>[10x]MKSLMKPNIKRVINATGVVINTNLGRAPLSKDVINFISEIANGYSNLEYNLEEGKRGSRIAHIEKYLNELTGAESSFVVNNNAGAVFLVLNTLA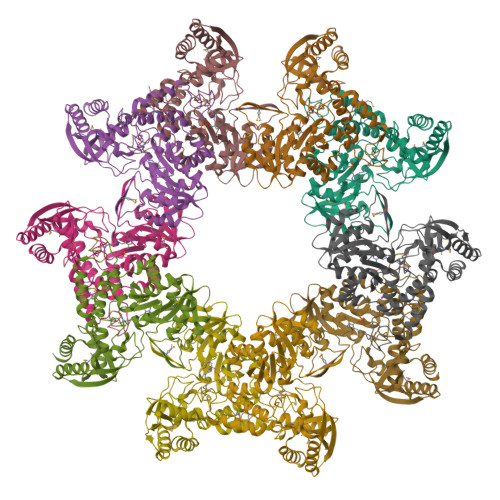EGKEVIISRGELVEIGGSFRIPDIMKKSGAILREVGTTNKTKVSDYEGAINQNTALLMKVHKSNFYMEGFVEEVKLEDLVKLGHKYGIPTYYDAGSGLLINLKEFGISVDEPNFRDCISLGIDLVSGSGDKLLGGPQAGIIVGKKNLIEKIKKNPIARALRIDKLTLSGLEMTLKLYFEKRYEDIPVIRMLTQDEKALRQKAKRLEKLLKDIPGLKISVIKDKAKPGGGSLPELELPTYCVAIRHDRLSSQELSRRLRLAEPPIVCRIREDQLLFDMRTVFHEDLKTIKKTLQELLSI In M. tuberculosis, the cell wall contains high levels of 3 → 3 (meso-Dap–meso-Dap) cross-links (approx. 80% at stationary phase), which are formed by the l,d-transpeptidases (Ldts) (ESI†).6 Evidence has emerged that LdtMt2, in particular, plays an important role in the virulence of M. tuberculosis, as disruption of the ldtMt2 gene results in altered morphology and inhibition of colony growth. Mechanistically, the Ldts differ from the PBPs through their use of a nucleophilic cysteine rather than serine during catalysis. Several β-lactam antibiotics, in particular carbapenems, have been shown to inhibit the activity of LdtMt2 and to have anti-TB activity. Such LdtMt2 inhibition involves covalent modification of the nucleophilic cysteine (Cys354), which reacts with β-lactam antibiotics to give (a) stable acyl–enzyme complex(es). Consistent with previous reports, the structure of LdtMt2 consists of two N-terminal immunoglobulin fold-related domains and a C-terminal catalytic domain.

To investigate the structural basis of LdtMt2 inhibition by ebselen, we carried out crystallographic studies. A comparison of our structures with reported LdtMt2 complex structures reveals variations in the conformation of the lid depending on the nature of the modification to Cys354. It appears that the hydrophobic residues of the lid (e.g., Tyr308, Met303, Tyr318, Thr320) can adjust to accommodate the group bonded to Cys354, apparently to optimise hydrophobic interactions. These results imply that the lid is conformationally dynamic, with the precise structure observed being related to the nature of modification of the nucleophilic Cys354.

>[2x]SMDLLVPKLTASVTDGAVGVTVDAPVSVTAADGVLAAVTMVNDNGRPVAGRLSPDGLRWSTTEQLGYNRRYTLNATALGLGGAATRQLTFQTSSPAHLTMPYVMPGDGEVVGVGEPVAIRFDENIADRGAAEKAIKITTNPPVEGAFYWLNNREVRWRPEHFWKPGTAVDVAVNTYGVDLGEGMFGEDNVQTHFTIGDEVIATADDNTKILTVRVNGEVVKSMPTSMGKDSTPTANGIYIVGSRYKHIIMDSSTYGVPVNSPNGYRTDVDWATQISYSGVFVHSAPWSVGAQGHTNTSHGCLNVSPSNAQWFYDHVKRGDIVEVVNTVGGTLPGIDGLGDWNIPWDQWRAGNAKA The first step of methanol metabolism, the oxidation with molecular oxygen to formaldehyde and hydrogen peroxide, is catalysed by alcohol oxidase (AOX) (EC 1.1.3.13) and occurs in specialized organelles, the peroxisomes, where H2O2 is decomposed by catalase. AOX is a member of the GMC (glucose–methanol–choline) oxidoreductase family and uses a non-covalently bound FAD cofactor. AOX catalyses the oxidation of small primary alcohols using a two-step mechanism, first a reductive half-reaction, where the substrate is oxidised while the FAD is reduced to FADH2, followed by an oxidative half-reaction, where the flavin is reoxidized by O2 and H2O2 is produced. AOX is with 663 amino acids larger than any of the other proteins, mainly due to a more than 70 residues long insert near the C-terminus that is thought to be involved in oligomerisation.

Here we present a cryo-EM map of Pichia pastoris alcohol oxidase at a resolution of 3.4 Å, which has allowed us to determine the structure of this protein. Unlike the other GMC family proteins, which act as monomers or dimers, AOX forms an octameric complex, consisting of two tetramers stacked face to face. The FAD density was also well resolved and indicated an FAD conformation typical for the GMC family. Structural elements unique for AOX are mostly located in the C-terminal half of the protein and include, apart from some short sections, a loop (364–392) including two α-helices connecting two β-strands of the 5-stranded parallel sheet (see below), a 75-residue insert (477–551) and a ~25 residue C-terminal extension (637–663). The AOX-specific inserts are located at the periphery of the monomer, where they mediate the inter-subunit contacts and form a tightly packed oligomer. The most significant oligomerisation module is the 75-residue insert 477–551, which is involved both in contacts within the tetrameric ring and in dimer contacts between rings. The FAD is buried deep inside the complex in an elongated conformation as in the other GMC family enzymes. In our model the space available for substrate molecules near the active site is restricted by large aromatic side chains, most strikingly Trp566, Phe98 and Phe402. In AOX, the dimer interface is close to the FAD isoalloxazine ring and the substrate binding pocket and the conserved side chain of His515 in the 75-residue AOX-specific oligomerisation loop appears to be part of the substrate binding pocket. Loss of this interaction in the monomer may be the cause of the observed inactivation of the FAD-containing monomer. The crystal contacts are formed by helix H12, which extends from the side of the octamer.

> MAIPEEFDILVLGGGSSGSCIAGRLANLDHSLKVGLIEAGENNLNNPWVYLPGIYPRNMKLDSKTASFYTSNPSPHLNGRRAIVPCANVLGGGSSINFMMYTRGSASDYDDFQAEGWKTKDLLPLMKKTETYQRACNNPDIHGFEGPIKVSFGNYTYPVCQDFLRASESQGIPYVDDLEDLVTAHGAEHWLKWINRDTGRRSDSAHAFVHSTMRNHDNLYLICNTKVDKIIVEDGRAAAVRTVPSKPLNPKKPSHKIYRARKQIVLSCGTISSPLVLQRSGFGDPIKLRAAGVKPLVNLPGVGRNFQDHYCFFSPYRIKPQYESFDDFVRGDAEIQKRVFDQWYANGTGPLATNGIEAGVKIRPTPEELSQMDESFQEGYREYFEDKPDKPVMHYSIIAGFFGDHTKIPPGKYMTMFHFLEYPFSRGSIHITSPDPYAAPDFDPGFMNDERDMAPMVWAYKKSRETARRMDHFAGEVTSHHPLFPYSSEARALEMDLETSNAYGGPLNLSAGLAHGSWTQPLKKPTAKNEGHVTSNQVELHPDIEYDEEDDKAIENYIREHTETTWHCLGTCSIGPREGSKIVKWGGVLDHRSNVYGVKGLKVGDLSVCPDNVGCNTYTTALLIGEKTATLVGEDLGYSGEALDMTVPQFKLGTYEKTGLARF> GSHMASDPKNLKDGQYDIAFKVLKDKTEEISMMNQYVVSPARLTVKDGKKYIAMTLKNSEWITKFQTEKNGGFADAKVVSEDKAANTRVVEFEANDLFAKLNAKVKVDID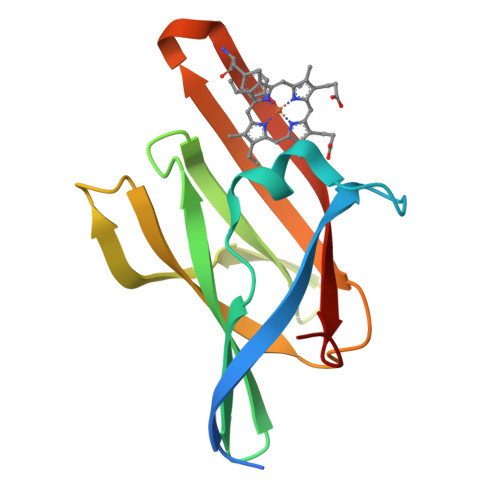SMNYHHFYDVQIQFDPTKI>[2x]MKKTFEKVYHLKLSIKGITPQIWRRIQVPENYTFLDLHKAIQAVMDWEDYHLHEFEMVNPKTGMLDKIGAEG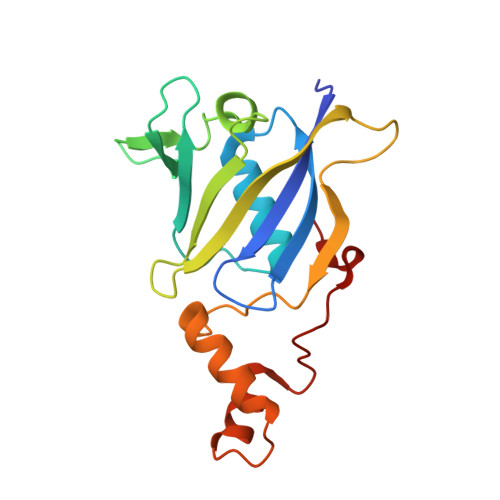DDFDAFGGPLVSEKKAKLSDYFTLENKEALYTYDFGDNWQVKVRLEKILPRKEGVEYPICTAGKRAAVPEDSGGVWGYEEMLEVLKDSEHEEYEDTVLWLGDDFDPEYFDPKDVSF> MSYKAQYTPGETRIAENRRKHMNPDYELRKLREISDEDLVKVLGHRNPGESYKSVHPPLDEMDFEEDIVRDLVEPIQGAKEGVRVRYI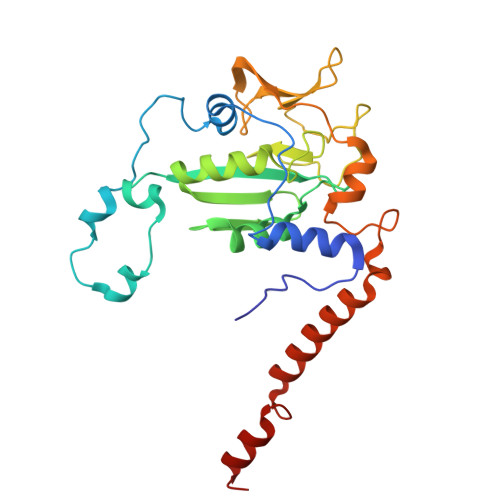QFADSMYNAPAQPYDRARTYMWRYRGVDTGTLSGRQVIEMRELDLEGVSKELVETELFDPATTGIRGATVHGHSLRLDENGLMFDALQRYVFDEETGHVVYVKEQVGRPLDEPVDMGQPLDEEELRKITTIYRKDNIAMRDDKEAIEVVENIHTGRTMGGFGMDVFKEDLRKRLGDD>MKHLEEKTLSTRQIFKGRYLKIEQDQVQAPDGRTYTREYILHPGAAMMIPLLPNGNVVMIHQYRHAVKKVFLEFPAGKRDHNEETLLTAKRELLEETGYEAKDWKFLTTIHPVIGYSNEHIDLYLARDLTHLEQRLDQGQFIEVVEVKPADLMQLVLEGKVSDVKTQIGAFWLDKFLRGEWN[2x]

Of particular interest is the Bdellovibrio bacteriovorus HD100 nucleoside diphosphate sugar (NDPS) hydrolase Bd3179 because it appears to have some of the characteristics of the Escherichia coli adenosine diphosphate ribose (ADPR) hydrolase and the guanosine diphosphate mannose (GDPM) hydrolase. Bd-NDPSase is a homodimer whose monomers are related by a non-crystallographic 2-fold axis. Each monomer comprises an N-terminal and a Nudix domain. Phosphate release assays revealed that among the nucleoside diphosphate sugars hydrolyzed by Bd-NDPSase, its highest relative activity was with GDPM.

Not surprisingly, substrate binding involves elements from both monomers. In fact, 46% of the buried ADPR surface in each active site is from the opposite monomer. Adenosine recognition involves hydrogen bonding by the E38’ (prime denotes a residue of the other monomer) main chain amide nitrogen and carbonyl oxygen to the adenosyl N1 and N6 respectively. R37’ and Y19 flank the nucleoside base though stacking interactions on opposite sides. As in Ec-NDPSase, Ec-ADPRase, and Mt-ADPRase, R64 of Bd-NDPSase forms a bidentate hydrogen bond through the guanidinium side chain with the β-phosphate oxygens O1β and O2β. In addition to nucleoside and phosphate recognition, Bd-NDPSase forms a network of hydrogen bonding interactions involving the three hydroxyl groups of the distal ribose. G115’ tethers both ends of an ADPR horseshoe conformation by hydrogen bonding to the hydroxyl at ribose C2 through its main chain amide nitrogen as well as to adenosine through the amide oxygen. The carboxylate of E119 makes a hydrogen bond with the hydroxyl at C3 and positions a water molecule to make a hydrogen bond to the hydroxyl on C2. The most distinguishing amino acid residues are K165 and D163, which form a bridge between the hydroxyl at C1 and the hydroxyl at the Cβ of T166. Interestingly, this network of interactions is also present in Ec-NDPSase, but not in Ec-ADPRase, suggesting that these residues may indeed be responsible for differentiation between GDPM and ADPR.> DYKDDDGAPLPQEYIRWGDAWAVGPVTIACLGALATLFVLGVFVRHNATPVVKASGRELCYILLGGVFLCYCMTFIFIAKPSTAVCTLRRLGLGTAFSVCYSALLTKTYRIARIFGAKALIVYGSTTGNTEYTAETIARELADAGYEVDSRDAASVEAGGLFEGFDLVLLGCSTWGDDSIELQDDFIPLFDSLEETGAQGRKVACFGCGDSSWEYFCGAVDAIEEKLKNLGAEIVQDGLRIDGDPRAARDDIVGWAHDVRGAIPRFISPASQVAICLALISGQLLIVVAWLVVEAPGTGKETAPERREVVTLRCNHRDASMLGSLAYNVLLIALCTLYAFKTRKCPENFNEAKFIGFTMYTTCIIWLAFLPIFYVTSSDYRVQTTTMCVSVSLSGSVVLGCLFAPKLYIILFQPQKNVVSHRAPTSRFGSAAA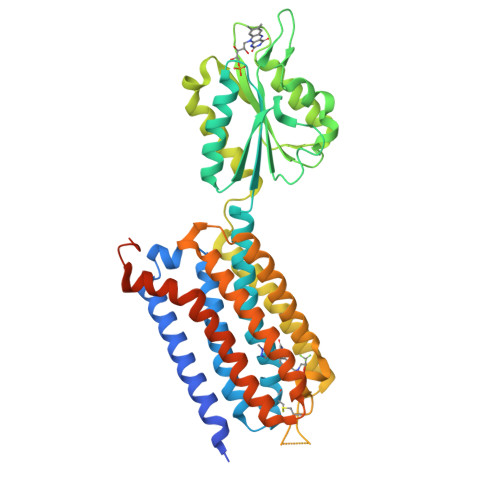RASSSEFLEVLFQ> MGSSHHHHHHHHSSGLEVLFQGPLGSHMNTRRQQAQNIRNN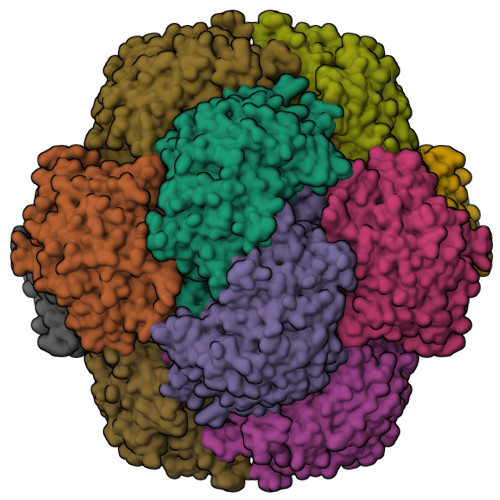AAELAANRPHPQHINNKEEYEYRRPKKDGNEPSHIANFTKGLPHDEHTGLLLNSADYDQFVLGIQSGDTTDFARTPLGPAELPKVHGCLSKQKIDCDDDHRSGFWKSQIAQGAAGGDGAKLRAWESAGAGLVFDLEGPDAQAVTMPPAPRLESPELTSEIAEVYSQALLRDIHFSQLRDPGLGDQVNACDSCPTQLSIYEAIDILNTVQIEGQNWFSANCCDLTDDEQARQRPLVTRQNIFRGIAPGDDVGPYLSQFLLIGNNALGGGVFGQEAGHIGYGAIRIDQRVRKATPCKDFMTNFETWLDVQNGADLRGLETYVDADPGKCREFPAYRVITTPRDLATYVHYDALYEAYLNACLILLGMGAPFDPGIPFQKPDVEDKQQGFAHFGGPQILTLVCEAATRGLKAVDFQKFNVHRRLRPEALGGLVDRYKHGKGAGDELKPVAALVEALENVGLLSKVVAHNQLQNQNLDRSGDPSSAGDNYFLPMAFPEGSPMHPSYGAGHATVAGACVTMLKAFFDHGWQLNLGMANGKYISYEPNQDGSSLQQVLLDCPLTVEGELNKIAANISIGRDWAGVHYFTDYIESLRLGEKIAIGILEEQKLTYGENFTMTVPLYDGGSIQI>[2x]MDQDYRARLVYPFSGAISPHADIVDQATLAWAAM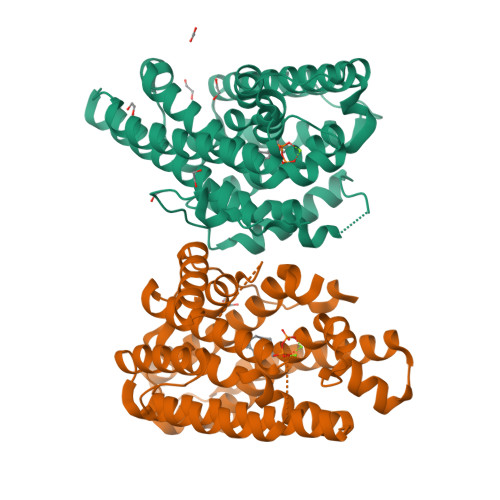FGLLTDSLRHKSRRLQYGLLAARAYPRADREMLQIAADWIAWLFFMDDQCDETGIGRDLQRMIALHERFLAILDGATPEAHDCALTYALADLRRRLALRAPDNWLRRFSEHVRLYFTANRWETVNRQRGATPNVATYCAARLFSGAVYACFDLIELAEQIELPFYARHHSIVQQLEQAANNIICWCNDVLSYPKEMQHGDRHNLVLVIQGEHQCSLPEAIDRALDLHAREVATFVRKRTCVPYFDAAVNTALEKYVTGLQFWICANRDWSLTATRYAPTHKSQEMVMAVAQQLEHHHHHH> GPRKAEIMESIKRLYPGSVYGRLIDLCQPTQKKYQIAVTKVLGKNMDAIIVDSEKTGRDCIQYIKEQRGEP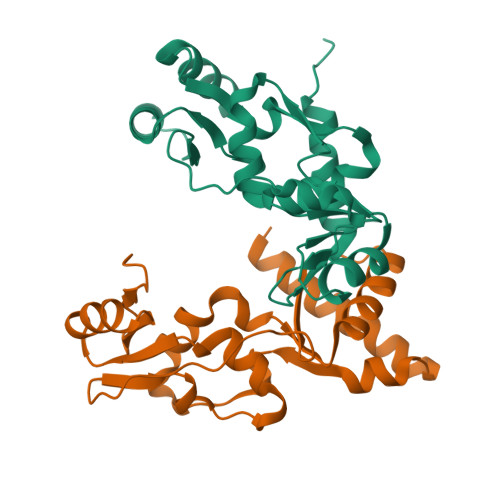ETFLPLDYLEVKPTDEKLRELKGAKLVIDVIRYEPPHIKKALQYACGNALVCDNVEDARRIAFGGHQRHKTVALDGTLFQKSGVISGGASDLKAKARRWDEKAVDKLK;> GPLGSGRPKQQLLRAATGKAILNGIDSINKVLDHFRRKGINQHVQNGYHGIVMNNFECEPAFYTCVEVTAGNRLFYHIVDSDEVSTKILMEFNKMNLPGEVTFLPLNKLDVRDTAYPETNDAIPMISKLRYNPRFDKAFKHVFGKTLICRSMEVSTQLARAFTMDCITLEGDQVSHRGALTGGYYDTRKSRLELQKDVRKA> MEFGFWSALYIFVLTCFLGYELITRVPVILHTPLMSGSNFIHGVVVVGAMVVLGHAETGLEKLIGFLGVILGAANAAGGYAVTVRMLEMFERKP;> MDLIQAAYFVVAILFIVGLKRMAHPTTAKSGIVWAGWGMVLAVLATFFWPGMGNFALILLALLLGSVVAWWAAVRVAMTDMPQMVAIYNGMGGGAAATIAAVELLKGAFENTGLMALAILGGLIGSVAFTGSLIAFAKL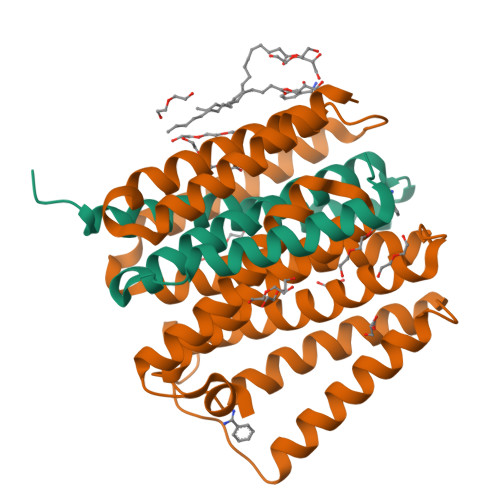QGIMKSRPILFPGQKAVNALVLALTVVIGLSLLWNDATASIVLFFLLALLFGVLMTLPIGGGDMPVAISFYNAFTGMAVGFEGFAVGNPALMVAGTLVGAAGTLLTVLMARAMNRSVWISVLVGG> MKKGHHHHHHENLYFQGGSLKLSAENESTPIQQLLEHFLRQLQRKDPHGFFAFPVTDAIAPGYSMII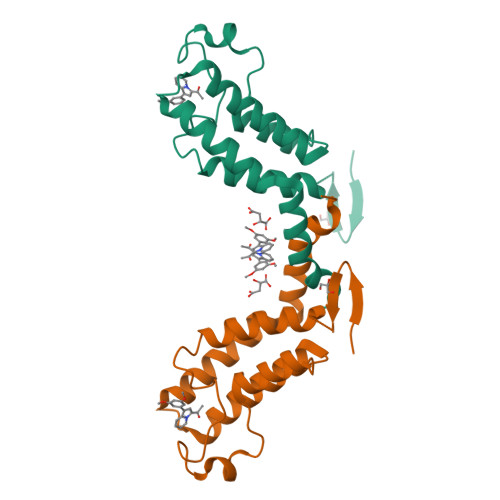KHPMDFGTMKDKIVANEYKSVTEFKADFKLMCDNAMTYNRPDTVYYKLAKKILHAGFKMMSKERLLALKRSMSFMQDMDFSQ>[2x]SSTCKVPRITTHYTIYPRDQDKRWEGVNMERFAEEADVVIVGAGPAGLSAATRLKQLAAQHEKDLRVCLVEKAAHIGAHTLSGACLDPRAFEELFPDWKEKGAPLNTPVTEDRFGILTEKYRIPVPILPGLPMNNHGNYVVRLGHLVSWMGEQAEALGVEVYPGYAAAEILFHEDGSVKGIATNDVGIQKDGAPKTTFERGLELHAKVTIFAEGCHGHLAKQLYKKFDLRANCEPQTYGIGLKELWVIDEKKWKPGRVDHTVGWPLDRHTYGGSFLYHLNEGEPLLALGFVVGLDYQNPYLSPFREFQRWKHHPSIKPTLEGGKRIAYGARALNEGGFQSIPKLTFPG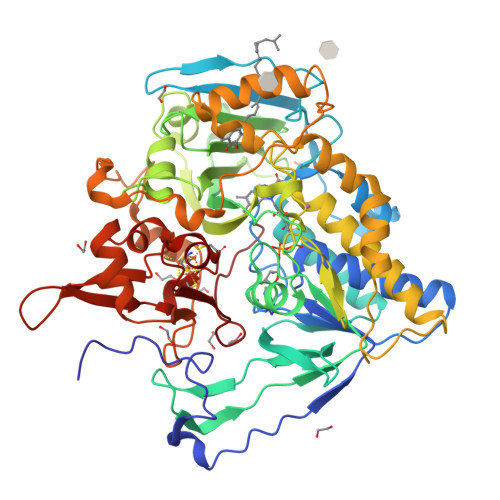GLLIGCSPGFMNVPKIKGTHTAMKSGTLAAESIFNQLTSENLQSKTIGLHVTEYEDNLKNSWVWKELYSVRNIRPSCHGILGVYGGMIYTGIFYWIFRGMEPWTLKHKGSDSDQLKPAKDCTPIEYPKPDGQISFDLLSSVALSGTNHEHDQPAHLTLKDDSVPVNRNLSIYDGPEQRFCPAGVYEFVPLEQGDGFRLQINAQNCVHCKTCDIKDPSQNINWVVPEGGGGPAYNGM4-(aminomethyl)-~{N}-[(2~{S})-1-oxidanylidene-3-phenyl-1-[[4-(1~{H}-1,2,3,4-tetrazol-5-yl)phenyl]amino]propan-2-yl]cyclohexane-1-carboxamide | C24 H29 N7 O2 | 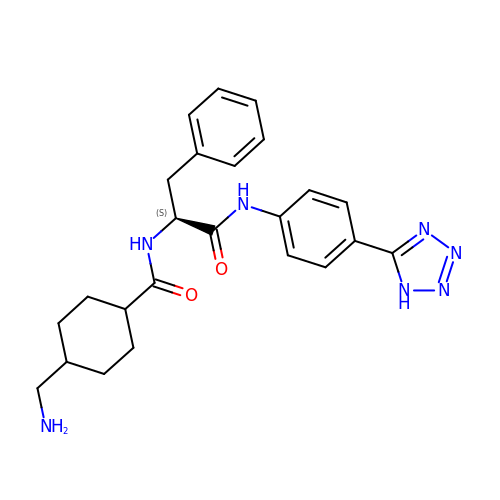WBOJRNOJLPGFJX-CUWPLCDZSA-N> GPGKRVYQIGSSSRDVQVCPRGAGAALRQEIEDKQLMVNNLTDELQDAIDEANPAEIANTSQQL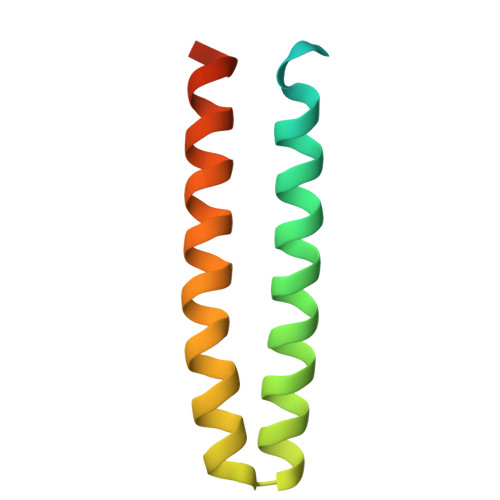RHARADLADLQRRFAVLRNEDRRINQ5-chloro-N~6~-(2,5-dimethoxybenzyl)quinazoline-2,4,6-triamine | C17 H18 Cl N5 O2 | 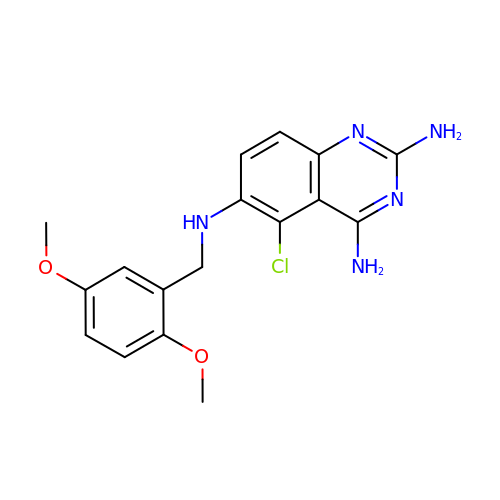ZQYDKYDSKVGDJP-UHFFFAOYSA-N> QAQITGRPEWIWLALGTALMGLGTLYFLVKGMGVSDPDAKKFYAITTLVAAIAFTMFLSMLLGYGLTMVPFGGEQNPIYWARYADWLFTTPLLLLDLALLVDADQGTILALVGADGIMIGTGLVGALTKVYSYRFVWWAISTAAMLYILYVLFFGFTSKAESMRPEVASTFKVLRNVTVVLWSAYPVVWLIGSEGAGIVPLNIETLLFMVLDVSAKVGFGLILLRSRAIFGEAEAPE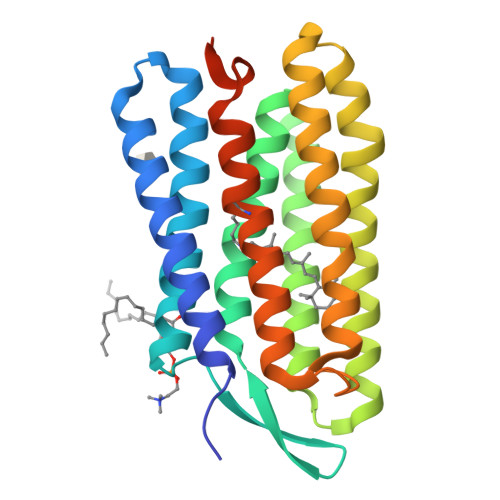PSAGDGAAATSD>GAGAYAYKTIKEDQKRYNERVMGLGLSPEEKQRRAIASATEGGSVPQIRAPSHVPFLLIGGGTAAFAAARSIRARDPGARVLIVSEDPELPYMRPPLSKELWFSDDPNVTKTLQFRQWNGKERSIYFQPPSFYVSAQDLPNIENGGVAVLTGKKVVHLDVRGNMVKLNDGSQITFEKCLIATGGTPRSLSAIDRAGAEVKSRTTLFRKIGDFRALEKISREVKSITVIGGGFLGSELACALGRKSQASGIEVIQLFPEKGNMGKILPQYLSNWTMEKVKREGVKVMPNAIVQSVGVSGGRLLIKLKDGRKVETDHIVTAVGLEPNVELAKTGGLEIDSDFGGFRVNAELQARSNIWVAGDAACFYDIKLGRRRVEHHDHAV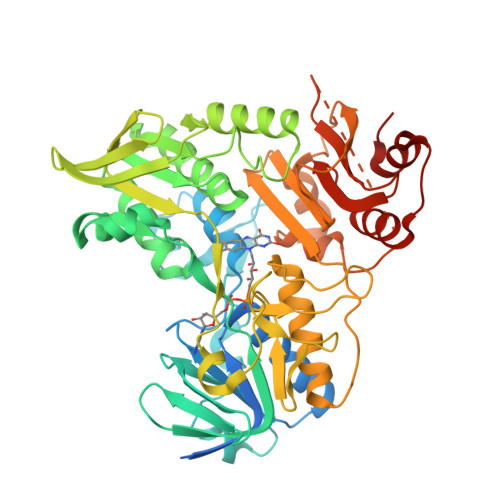VSGRLAGENMTGAAKPYWHQSMFWSDLGPDVGYEAIGLVDSSLPTVGVFAKATAQDNPKSATEQSGTGIRSESETESEASEITIPPSAPAVPQVPVEGEDYGKGVIFYLRDKVVVGIVLWNVFNRMPIARKIIKDGEQHEDLNEVAKLFNIHED[4x]2,5-DIMETHYLANILINE | C8 H11 N | 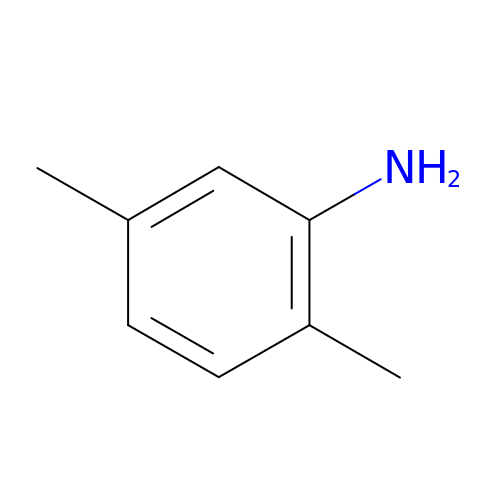VOWZNBNDMFLQGM-UHFFFAOYSA-N>MKHVPPTVLVWFRNDLRLHDHEPLHRALKSGLAITAVYCYDPRQFAQTHQGFAKTGPWRSNFLQQSVQNLAESLQKVGNKLLVTTGLPEQVIPQIAKQINAKTIYYHREVTQEELDVERNLVKQLTILGIEAKGYWGSTLCHPEDLPFSIQDLPDLFTKFRKDIEKKKISIRPCFFAPSQLLPSPNIKLELTAPPPEFFPQINFDHRSVLAFQGGETAGLARLQDYFWHGDRLKDYKETRNGMVGADYSSKFSPWLALGCLSPRFIYQEVKRYEQERVSNDSTHWL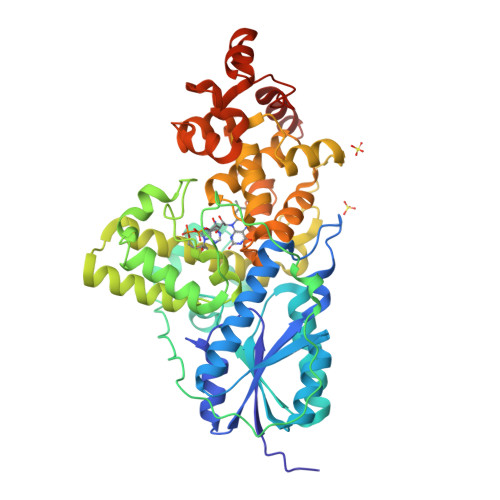IFELLWRDFFRFVAQKYGNKLFNRGGLLNKNFPWQEDQVRFELWRSGQTGYPLVDANMRELNLTGFMSNRGRQNVASFLCKNLGIDWRWGAEWFESCLIDYDVCSNWGNWNYTAGIGNDARDFRYFNIPKQSQQYDPQGTYLRHWLPELKNLPGDKIHQPWLLSATEQKQWGVQLGVDYPRPCVNFHQSVEARRKIEQMGVIA[2x]>GSHMPMYEVQWKVVEESNGNNYSYIDPTQLPYDHKWEFPRNRLSFGKTLGAGAFGKVVEATAQGLIKSDAAMTVAVKMLKPSAHSTEREALMSELKVLSYLGNHENIVNLLGACTHGGPTLVITEYCCYGDLLNFLRRKRDEFVPYKVAPEDLYKDFLTLEHLLSFSYQVAKGMAFLASKNCIHRDLAARNILLTHGNITKICDFGLARDIKNDSNYVDKGNARLPVKWMAPESIFNSVYTFESDVWSYGIFLWELFSLGSSPYPGM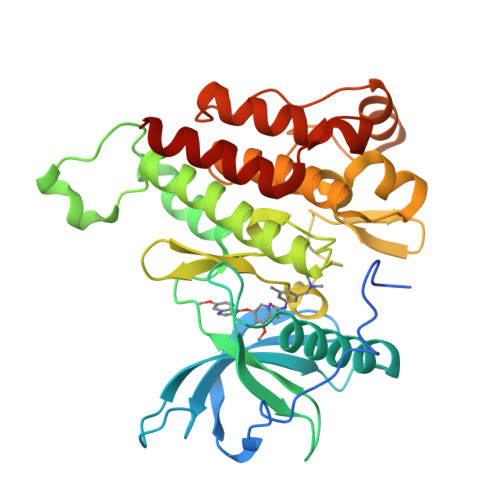PVDSKFYKMIKEGFRMSSPEYAPAEMYDIMKTCWDADPDKRPTFKQIVQDIEKQISESTNH[2x]>[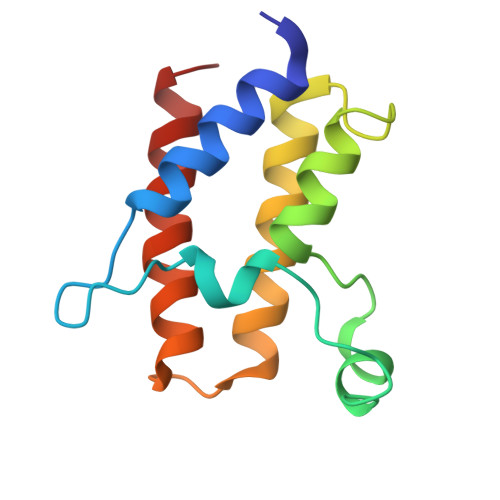4x]SLGIFPTVEKLVEEMREQLDEVDSHPRTSIFEKLPSKRDYPDYFKVIEKPMAIDIILKNCKNGTYKTLEEVRQALQTMFENARFYNEEGSWVYVDADKLNEFTDEWFKEHSS>MKKIIYIATIGITLLTTSCDDFLDRQVPQGIVTGDQIASPEYVDNLVISAYAIWATGDDINSSFSLWNYDVRSDDCYKGGSGTEDGGVFNALEISKGINTTDWNINDIWKRLYQCITRANTALQSLDQMDEKTYPLKNQRIAEMRFLRGHAHFMLKQLFKKIVIVNDENMEPDAYNELSNTTYTNDEQWQKIADDFQFAYDNLPEVQIEKGRPAQAAAAAYLAKTYLYKAYRQDGADNALTGINEEDLKQVVKYTDPLIMAKGGYGLETDYSMNFLPQYENGAESVWAIQYSINDGTYNGNLNWGMGLTTPQILGCCDFHKPSQNLVNAFKTDSQGKPLFSTYDNENYEVATDNVDPRLFHTVGMPGFPYKYNEGYIIQKNDDWSRSKGLYGYYVSLKENVDPDCDCLKKGSYWASSLNHIVIRYADVLLMRAEALIQLNDGRITDAISLINEVRSRAAGSTMLIFNYKEDYGVNFKVTPYDLKAYAQDEAMKMLKWERRVEFGMESSRFFDLVRWGEAKDVINAYYVTEASRCSIYKNAGFTENKNEYLPVPFEQISASNGNYTQNFGWAAAAHHHHHH[2x];>MPGIMKNKKLLCSVCFLFAFMSALWGQNITVKGNVTSKTDGQPIIGASVVETTATTNGTITDFDGNFTLSVPVNSTLKITYIGYKPVTVKAAAIVNVLLEEDTQMVDEVVVTGYTTQRKADLTGAVSVVKVDEIQKQGENNPVKALQGRVPGMNITADGNPSGSATVRIRGIGTLNNNDPLYIIDGVPTKAGMHELNGNDIESIQVLKDAASASIYGSRAANGVIIITTKQGKKGQIKINFDASVSASMYQSKMNVLNTEQYGRAMWQAYVNDGENPNGNALGYAYNWGYNADGNPVLYGMTLSKYLDSKNTMPVADTDWFDEITRTGVIQQYNLSVSNGSEKGSSFFSLGYYKNLGVIKDTDFDRFSARMNSDYKLIDDILTIGQHFTLNRTSEVQAPGGIIETALDIPSAIPVYASDGSWGGPVGGWPDRRNPRAVLEYNKDNRYTYWRMFGDAYVNLTPFKGFNLRSTFGLDYANKQARYFTYPYQEGTQTNNGKSAVEAKQEHWTKWMWNAIATYQLEVGKHRGDVMIGMELNREDDSHFSGYKEDFSILTPDYMWPDAGSGTAQAYGAGEGYSLVSFFGKMNYSYADRYLLSLTLRRDGSSRFGKNHRYATFPSVSLGWRITQENFMKELTWLDDLKLRASWGQTGNQEISNLARYTIYAPNYGTTDSFGGQSYGTAYDITGSNGGGVLPSGFKRNQIGNDNIKWETTTQTNVGIDFSLFKQSLYGSLEYYYKKATDILTEMAGVGVLGEGGSRWINSGAMKNQGFEFNLGYRNKTAFGLTYDLNGNISTYRNEILELPETVAANGKFGGNGVKSVVGHTYGAQVGYIADGIFKSQDEVDNHATQEGAAVGRIRYRDIDHNGVIDERDQNWIYDPTPSFSY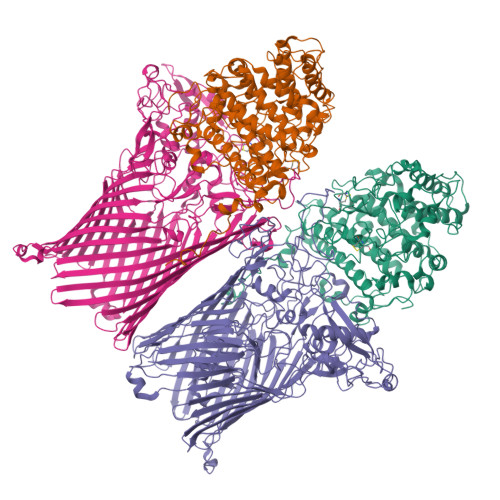GLNIYLEYKNFDLTMFWQGVQGVDIISDVKKKSDFWSASNVGFLNKGTRLLNAWSPTNPNSDIPALTRSDTNNEQRVSTYFVENGSFLKLRNIQLGYTVPAVISKKMRMDRLRFYCSAQNLLTIKSKNFTGEDPENPNFSYPIPVNITFGLNIGF[2x]> GPLGSQMTRQARRLYVGNIPFGITEEAMMDFFNAQMRLGGLTQA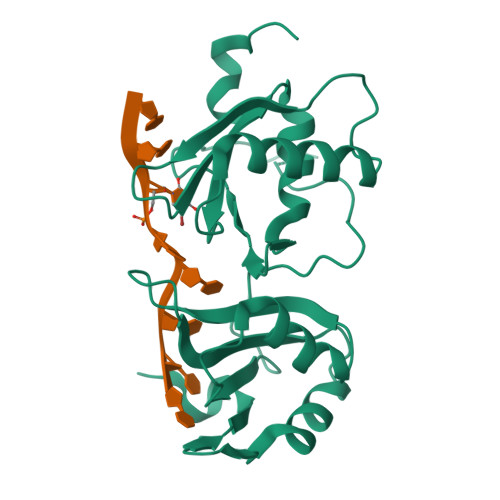PGNPVLAVQINQDKKFAFLEFRSVDETTQAMAFDGIIFQGQSLKIRRPHDYQPLPGMSENPSVYVPGVVSTVVPDSAHKLFIGGLPNYLNDDQVKELLTSFGPLKAFNLVKDSATGLSKGYAFCEYVDINVTDQAIAGLNGMQLGDKKLLVQRASVGAKN>[2x]SNAMSKLPENFLWGGAVAAHQLEGGWQEGGKGISVADVMTAGRHGVAREITAGVLEGKYYPNHEAIDFYHHYKEDVKLFAEMGFKCFRTSIAWTRIFPKGDEAEPNE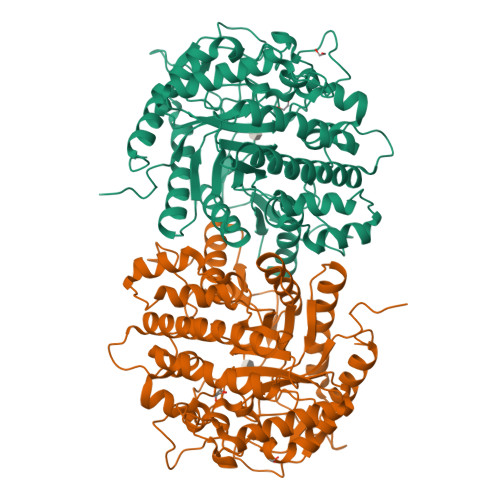AGLQFYDDLFDECLKYGIEPVVTLSHFELPYHLVTEYGGFTNRKVIDFFVHFAEVCFRRYKDKVKYWMTFNEINNQANYQEDFAPFTNSGIVYKEGDDREAIMYQAAHYELVASARAVKIGHAINPNLNIGCMVAMCPIYPATCNPKDILMAQKAMQKRYYFADVHVHGFYPEHIFKYWERKAIKVDFTERDKKDLFEGTVDYIGFSYYMSFVIDAHRENNPYYDYLETEDLVKNPYVKASDWDWQIDPQGLRYALNWFTDMYHLPLFIVENGFGAIDQVEADGMVHDDYRIDYLGAHIKEMIKAVDEDGVELMGYTPWGCIDLVSAGTGEMRKRYGFIYVDKDDEGKGTLKRSPKLSFNWYKEVIASNGDDI>[3x]YFQGMQLRFARLSEHATAPTRGSARAAGYDLYSAYDYTIPPMEKAVVKTDIQIALPSGCYGRVAPRSGLAAKHFIDVGAGVIDEDYRGN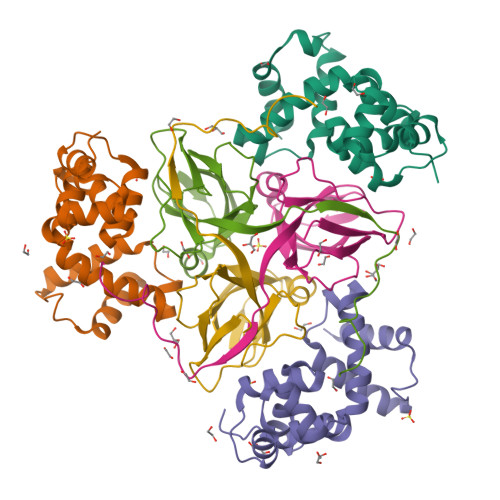VGVVLFNFGKEKFEVKKGDRIAQLICERIFYPEIEEVQALDDTERGSGGFGSTGKN;>[3x]MEGAGQMAELPTHYGTIIKTLRKYMKLTQSKLSERTGFSQNTISNHENGNRNIGVNEIEIYGKGLGIPSYILHRISDEFKEKGYSPTLNDFGKFDKMYSYVNKAYYNDGDIYYSSYDLYDETIKLLELLKESKINVNDIDYDYVLKLYKQILSTDT> GXGU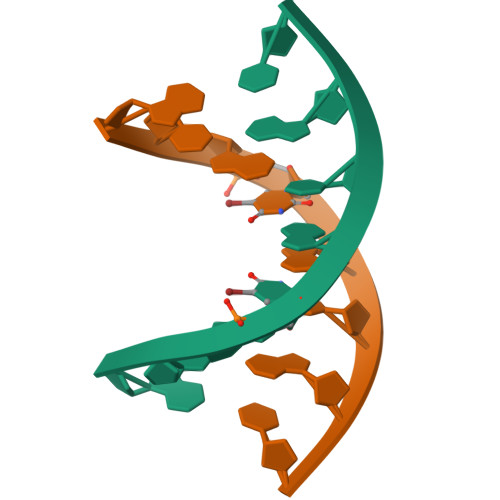ACAC> SMKINFLRNKHKIHVQGTDLPDPIATFQQLDQEYKINSRLLQNILDAGFQMPTPIQMQAIPVMLHGRELLASAPTGSGKTLAFSIPILMQLKQPANKGFRALIISPTRELASQIHRELIKISEGTGFRIHMIHKAAVAAKKFGPKSSKKFDILVTTPNRLIYLLKQDPPGIDLASVEWLVVDESDKLFEDGKTGFRDQLASIFLACTSHKVRRAMFSATFAYDVEQWCKLNLDNVISVSIGARNS

DExD/H-box RNA helicases, from virus and bacteria to eukaryotes, play important roles in processes including ribosome biogenesis, RNA processing and folding, ribonucleoprotein (RNP) remodeling, RNA nuclear export, the regulation of RNA translation and transcription, and nonsense-mediated RNA decay. DExD/H-box proteins often contain accessory regulatory domains and localization modules, but their cores consist of two RecA-like domains joined by a short flexible linker. The N-terminal domain is commonly referred to as conserved domain-1, or DEAD-domain, and the C-terminal domain as conserved domain-2, or helicase domain. Both domains contribute to the binding site for RNA substrates and both contribute to ATP hydrolysis. We used X-ray crystallography to determine the structures of the DEAD-domains of DDX2A, DDX2B, DDX5, DDX10, DDX18, DDX20, DDX47, DDX52, and DDX53, as well as the helicase domains of DDX25 and DDX41.

DDX52 (Rok1) is required for the release of snR30 (small nucleolar RNA-30) from pre-ribosomes. snR30 is one of three snoRNAs that are critical for pre-rRNA processing in yeast. DDX52 ATPase activity is important for optimal pre-ribosomal RNA processing, but not essential for release of snR30. In the crystal complexes with either ADP or AMP the loop closes up, resulting in a shift in Cα-atom positions by up to 3.5 Å between the ATP- and the AMP-states, or by up to 2.5 Å between the ADP- and the AMP-state. Thus the conformation of the P-loop is determined by the nucleotide phosphates, and longer phosphate tails result in a more open loop.> SHMLRPVETPTREIKKLDGLWAFSLDRENCGIDQRWWESALQESRAIAVPGSFNDQFADADIRNYAGNVWYQREVFIPKGWAGQRIVLRFDAVTHYGKVWVNNQEVMEHQGGYTPFEADVTPYVIAGKSVRITVCVNNELNWQTIPPGMVITDENGKKKQSYFHDFFNYAGIHRSVMLYTTPNTWVDDITVVTHVAQDCNHASVDWQVVANGDVSVELRDADQQVVATGQGTSGTLQVVNPHLWQPGEGYLYELCVTAKSQTECDIYPLRVGIRSVAVKGEQFLINHKPFYFTGFGRHEDADLRGKGFDNVLMVHDHALMDWIGANSYRTSHYPYAEEMLDWADEHGIVVIDETAAVGFNLSLGIGFEAGNKPKELYSEEAVNGETQQAHLQAIKELIARDKNHPSVVMWSIANEPDTRPQGAREYFAPLAEATRKLDPTRPITCVNVMFCDAHTDTISDLFDVLCLNRYYGWYVQSGDLETAEKVLEKELLAWQEKLHQPIIITEYGVDTLAG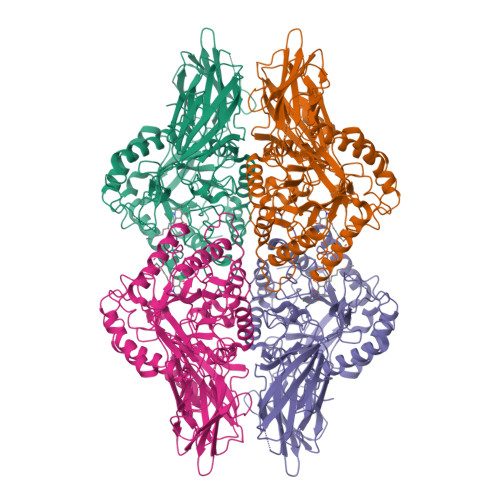LHSMYTDMWSEEYQCAWLDMYHRVFDRVSAVVGEQVWNFADFATSQGILRVGGNKKGIFTRDRKPKSAAFLLQKRWTGMNFGEKPQQGGKQ;> RPVETPTREIKKLDGLWAFSLDRENCGIDQRWWESALQESRAIAVPGSFNDQFADADIRNYAGNVWYQREVFIPKGWAGQRIVLRFDAVTHYGKVWVNNQEVMEHQGGYTPFEADVTPYVIAGKSVRITVCVNNELNWQTIPPGMVITDENGKKKQSYFHDFFNYAGIHRSVMLYTTPNTWVDDITVVTHVAQDCNHASVDWQVVANGDVSVELRDADQQVVATGQGTSGTLQVVNPHLWQPGEGYLYELCVTAKSQTECDIYPLRVGIRSVAVKGEQFLINHKPFYFTGFGRHEDADLRGKGFDNVLMVHDHALMDWIGANSYRTSHYPYAEEMLDWADEHGIVVIDETAAVGFNLSLGIGFEAGNKPKELYSEEAVNGETQQAHLQAIKELIARDKNHPSVVMWSIANEPDTRPQGAREYFAPLAEATRKLDPTRPITCVNVMFCDAHTDTISDLFDVLCLNRYYGWYVQSGDLETAEKVLEKELLAWQEKLHQPIIITEYGVDTLAGLHSMYTDMWSEEYQCAWLDMYHRVFDRVSAVVGEQVWNFADFATSQGILRVGGNKKGIFTRDRKPKSAAFLLQKRWTGMNFGEKPQQGGKQ> NDKVYEN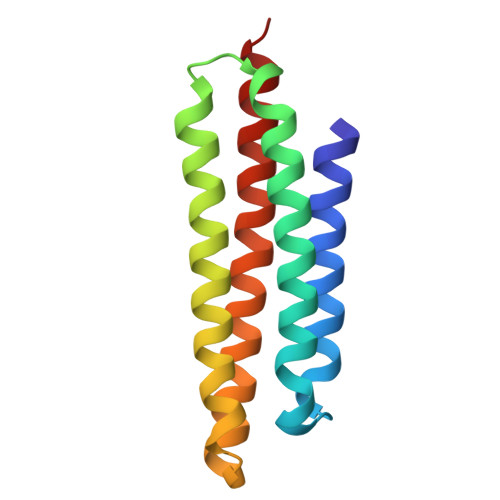VTGLVKAVIEMSSKIQPAPPEEYVPMVKEVGLALRTLLATVDETIPALPASTHREIEMAQKLLNSDLGELISKMKLAQQYVMTSLQQEYKKQMLTAAHALAVDAKNLLDVIDQARLKML>MLASSPSGHTNPVLSGAPLSINVVADIGRQRLIPSLTDDEQVLNRVHACRDVVQKAVRNNERIYGITTGFGGMSDIPIPPQHVAQTQDNLLAFLSTSTGASLDPRHVRAAMALRANVLLQGRSGVRLELIERLVEFLRQDAIPVVCDLGSIGASGDLVPLGVIARSIIGHPSTTQVKYQGEQADSHDVLQQLNYSALQLEAKEGLALVNGTSFSSAIAANCVFESQRLLSLSLVLQSIMVRALGGHPEAFHPFVDENKPHPGQGWSAQMMRDLLSYSPNDSKRNGDLAQDRYSLRCLAQYFAPIVEGIAQISQSISTEMNAVSDNPLIDVDTGRFHQSGNFLGQYVAMSMDQLRRHLGLLAKHLDVQIAQLVAPAFNNGLPASLRGNSSRPFNMGLKGLQITGNSIMPLLTYLGNPLTEHFPTHAEEFNQNINGLSWGSANLAWRSVQLFQHYLSVASIFAVQAIDLRAGLEADHCDGRELLGETATELYETVYDLLERNCGQESPFLFND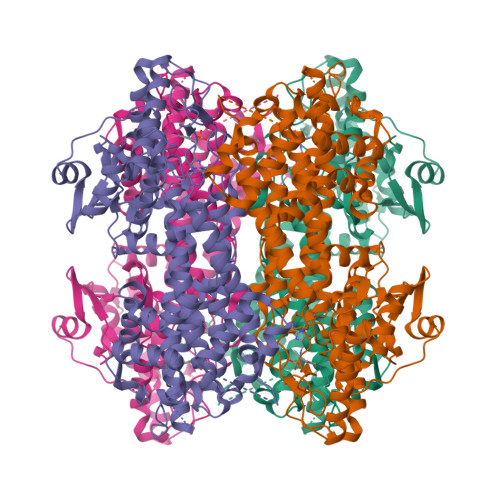DEQSLEVDLQMLNGDLAGAGRMHEAVSSVTDSFLAEFCESGGGLEVLFQGPGGSSGSGHHHHHHHHH[4x]> GCGTG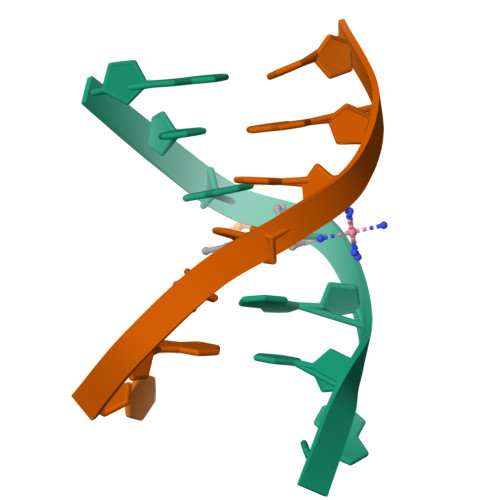CG;> CGCACGC> ADPGGSHHHHHSRK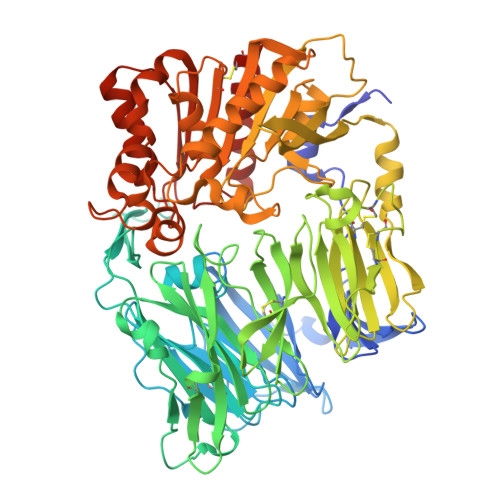TYTLTDYLKNTYRLKLYSLRWISDHEYLYKQENNILVFNAEYGNSSVFLENSTFDEFGHSINDYSISPDGQFILLEYNYVKQWRHSYTASYDIYDLNKRQLITEERIPNNTQWVTWSPVGHKLAYVWNNDIYVKIEPNLPSYRITWTGKEDIIYNGITDWVYEEEVFSAYSALWWSPNGTFLAYAQFNDTEVPLIEYSFYSDESLQYPKTVRVPYPKAGAVNPTVKFFVVNTDSLSSVTNATSIQITAPASMLIGDHYLCDVTWATQERISLQWLRRIQNYSVMDICDYDESSGRWNCLVARQHIEMSTTGWVGRFRPSEPHFTLDGNSFYKIISNEEGYRHICYFQIDKKDCTFITKGTWEVIGIEALTSDYLYYISNEYKGMPGGRNLYKIQLSDYTKVTCLSCELNPERCQYYSVSFSKEAKYYQLRCSGPGLPLYTLHSSVNDKGLRVLEDNSALDKMLQNVQMPSKKLDFIILNETKFWYQMILPPHFDKSKKYPLLLDVYAGPCSQKADTVFRLNWATYLASTENIIVASFDGRGSGYQGDKIMHAINRRLGTFEVEDQIEAARQFSKMGFVDNKRIAIWGWSYGGYVTSMVLGSGSGVFKCGIAVAPVSRWEYYDSVYTERYMGLPTPEDNLDHYRNSTVMSRAENFKQVEYLLIHGTADDNVHFQQSAQISKALVDVGVDFQAMWYTDEDHGIASSTAHQHIYTHMSHFIKQCFSLP>GANMAGRSMQAARCPTDELSLSNCAVVSEKDYQSGQHVIVRTSPNHKYIFTLRTHPSVVPGSVAFSLPQRKWAGLSIGQEIEVALYSFDKAKQCIGTMTIEIDFLQKKNIDSNPYDTDKMAAEFIQQFNNQAFSVGQQLVFSFNDKLFGLLVKDIEAMDPSILKGEPASGKRQKIEVGLVVGNSQVAFEKAENSSLNLIGKAKTKENRQSIINPDWNFEKMGIGGLDKEFSDIFRRAFASRVFPPEIVEQMGCKHVKGILLYGPPGCGKTLLARQIGKMLNAREPKVVNGPEILNKYVGESEANIRKLFADAEEEQRRLGANSGLHIIIFDEIDAICKQRGSMAGSTGVHDTVVNQLLSKIDGVEQLNNILVIGMTNRPDLIDEALLRPGRLEVKMEIGLPDEKGRLQILHIHTARMRGHQLLSADVDIKELAVETKNFSGAELEGLVRAAQSTAMNRHIKASTKVEVDMEKAESLQVTRGDFLASLENDIKPAFGTNQEDYASYIMNGIIKWGDPVTRVLDDGELLVQQTKNSDRTPLVSVLLEGPPHSGKTALAAKIAEESNFPFIKICSPDKMIGFSETAKCQAMKKIFDDAYKSQLSCVVVDDIERLLDYVPIGPRFSNLVLQALLVLLKKAPPQGRKLLIIGTTSRKDVLQEMEMLNAFSTTIHVPNIATGEQLLEALELLGNFKDKERTTIAQQVKGKKVWIGIKKLLMLIEMSLQMDPEYRVRKFLALLREEGASPLDFD[6x];>[2x]MKDRTQELRTAKDSDDDDDVTVTVDRDRFMDEFFEQVEEIRGFIDKIAENVEEVKRKHSAILASPNPDEKTKEELEELMSDIKKTANKVRSKLKSIEQSIEQEEGLNRSSADLRIRKTQHSTLSRKFVEVMSEYNATQSDYRERCKGRIQRQLEITGRTTTSEELEDMLESGNPAIFASGIIMDSSISKQALSEIETRHSEIIKLENSIRELHDMFMDMAMLVESQGEMIDRIEYNVEHAVDYVERAVSDTKKAVKYQSKARRKKIM;>MGSSHHHHHHSQDPNSMAEDADMRNELEEMQRRADQLADESLESTRRMLQLVEESKDAGIRTLVMLDEQGEQLERIEEGMDQINKDMKEAEKNLTDLGKFAGLAVAPANKLKSSDAYKKAWGNNQDGVVASQPARVVDEREQMAISGGFIRRVTNDARENEMDENLEQVSGIIGNLRHMALDMGNEIDTQNRQIDRIMEKADSNKTRIDEANQRATKMLGSGGMDTSGKQAEAMALLAEAERKVKNSQSFFSGLFGGSSKIEEACEIYARAANMFKMAKNWSAAGNAFCQAAQLHLQLQSKHDAATCFVDAGNAFKKADPQEAINCLMRAIEIYTDMGRFTIAAKHHISIAEIYETELVDVEKAIAHYEQSADYYKGEESNSSANKCLLKVAGYAAQLEQYQKAIDIYEQVGTSAMDSPLLKYSAKDYFFKAALCHFCIDMLNAKLAVQKYEELFPAFSDSRECKLMKKLLEAHEEQNVDSYTESVKEYDSISRLDQWLTTMLLRIKKTIQGDEEDLR[2x];>[4x]GMDTSGKQAEAMALLAEAERKVKNSQSFFSGLFGGSSKIEEACEIYARAANMFKMAKNWSAAGNAFCQAAQLHLQLQSKHDAATCFVDAGNAFKKADPQEAINCLMRAIEIYTDMGRFTIAAKHHISIAEIYETELVDVEKAIAHYEQSADYYKGEESNSSANKCLLKVAGYAAQLEQYQKAIDIYEQVGTSAMDSPLLKYSAKDYFFKAALCHFCIDMLNAKLAVQKYEELFPAFSDSRECKLMKKLLEAHEEQNVDSYTESVKEYDSISRLDQWLTTMLLRIKKTIQGDEEDLR

The membrane-anchored SNARE (soluble N-ethylmaleimide-sensitive factor acceptor protein receptor) proteins provide the energy to drive membrane fusion in various cellular contexts, such as intracellular trafficking and exocytosis. Supercomplexes of NSF, α-SNAP, and either a syntaxin tetramer or one of two binary complexes of syntaxin—SNAP-25 reveal atomic details of SNARE processing and show how sequential ATP hydrolysis drives disassembly. NSF comprises three structured domains connected by flexible linkers—the adapter N-domain followed by the D1 and D2 AAA+ domains. Six NSF protomers come together to form the active form of the enzyme, a homo-hexamer.

Following 3D classification, 41% of particles formed a complete complex, all of which have ordered ɑ-SNAP—SNARE spire density and differ largely by spire pose. Substrate-bound reconstructions reveal a flattened D1 ring in closer proximity to the D2 ring and a strikingly different ɑ-SNAP—SNARE spire structure than observed in the 21bin20S complex under non-hydrolyzing conditions. Again, syntaxin is bound within the pore of the D1 ring. We observed a nearly symmetric ɑ-SNAP—SNARE subcomplex comprising four ɑ-SNAP molecules coating a four-helix bundle. Even without further processing, this structure was recognizable as a parallel 2:2 syntaxin—SNAP-25 sub-complex formed by two syntaxin H3 SNARE domains and two SNAP-25 SN1 SNARE domains; this binary 2:2 configuration was previously observed in crystal structures of syntaxin-1 H3 and SNAP-25 SN1 domains and was unexpected as we prepared the complex with full-length proteins, implying that two independent SNAP-25 molecules contribute their SN1 SNARE domains to this complex. Presumably, disassembly of the binary 2:1 complex had occurred and was followed by reassembly of the 2:2 binary complex before vitrification. Of the five 22bin20S classes with the 2:2 binary SNARE complex, all are found with syntaxin in the D1 pore, while two are observed with the N-terminus of the SNAP-25 SN1 domain in the pore. Most strikingly, no SNARE substrate-bound classes show an F protomer as fully engaged as those in non-hydrolyzing classes; in all but one class, F is ADP bound, SNARE substrate disengaged, and sits between engaged A and E protomers. Three distinctive “grips” are observed in the case of the classes with the 2:1 syntaxin—SNAP-25 complex identified under non-hydrolyzing conditions (top), and two are observed in the case of the classes with the 2:2 syntaxin—SNAP-25 SNARE complex identified under hydrolyzing conditions (bottom).> MARMGDFGVVDYTSLMALAPRSKNFLELLGVFSESNTRYIDSRYAEFEREEKGVTKMNAMARGGSRKYIGSEKARKEIIEVPFAPLDGVTVASEVEAFRQYGTESQTASVEALVQRKIEHIQRSHGIYIRDCQYTALLKDKILAEDEDGNEITALAKNFSTLWGVSRKTGAINTTTAVNPFSVLATKRQEIIDSMGENNGFTSMVVLCTTRDFNAIVDHPDVRAAYEGRDGGAEYLTRRLGDAVDFQVFTHKGVTLVEDTSGKLTDGSAYMFPLGVQDMFQAVYAPADSTDHVNTISQGSYLFLNAGENWRRDVIESEVSYACMVTRSELICDLTITV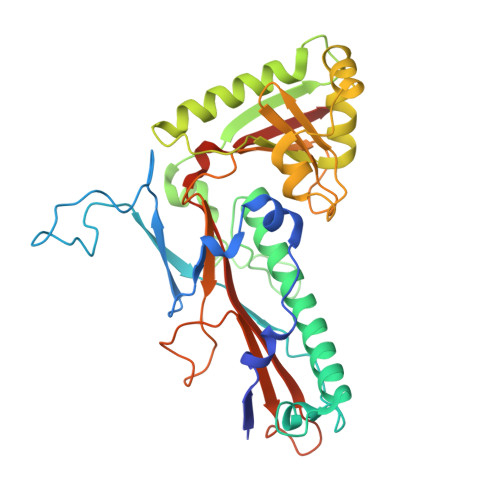AHHHHHH> MSNLVKEKAPVFPISKVKKIAKCDPEYVITSNVAISATAFAAELFVQNLVEESLVLAQLNSKGKTSLRLSLNSIEECVEKRDNFRFLEDAIKQLKKNSALDKKRELNMQPGRSDQEVVIEEPELHEDDGVEEEEEEDEVSEEEEPVHNEELLDDSKDQQNDKSTRSVASLLSRFQYK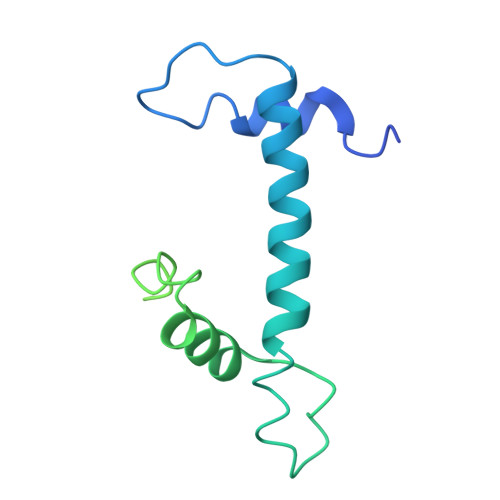SALDVGEHSDSSDIEVDHTKSTDP>[2x]II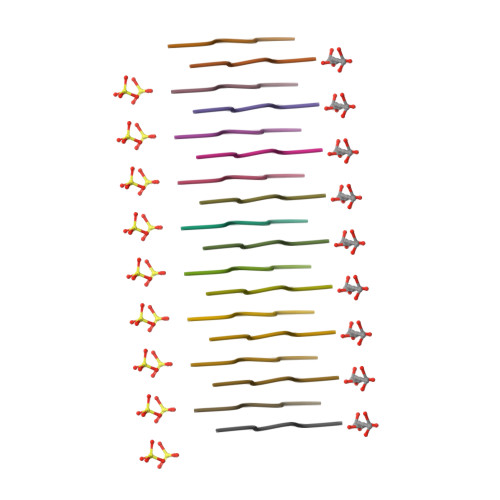KIIK>MNNLYRDLAPITESAWAEIELEATRTFKRHIAGRRVVDVSGPNGPTTASVSTGHLLDVSPPGDGVIAHLRDAKPLVRLRVPFTVARRDID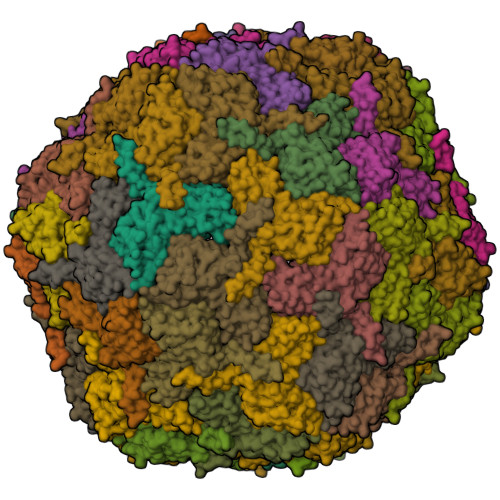DVERGSQDSDWDPVKDAAKKLAFVEDRAIFEGYAAASIEGIRSSSSNPALALPDDAREIPDVIAQALSELRLAGVDGPYSVLLSAETYTKVSETTAHGYPIREHINRLVDGEIIWAPAIDGAFVLSTRGGDFDLQLGTDVSIGYLSHDAEVVHLYMEETMTFLCYTAEASVALTPELWSHPQFEK[60x]>GKLHVGKMGFVVTMLKLIQKKLLDKTCDQVMEFSWSALW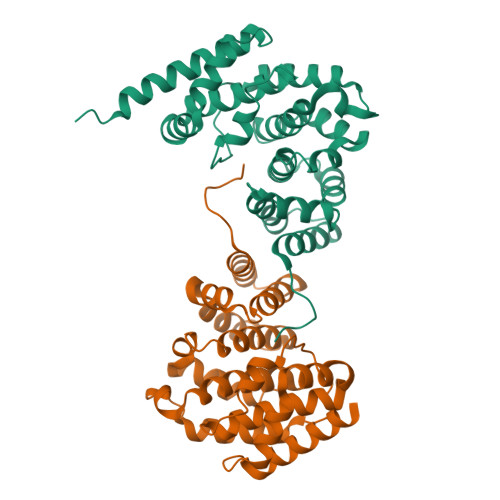NITDETPDNCEMFLNFNGMKLFLDCLKEFPEKQELHRNMLGLLGNVAEVKELRPQLMTSQFISVFSNLLESKADGIEVSYNACGVLSHIMFDGPEAWGVCEPQREEVEERMWAAIQSWDINSRRNINYRSFEPILRLLPQGISPVSQHWATWALYNLVSVYPDKYCPLLIKEGGMPLLRDIIKMATARQETKEMARKVIEHCSNFKEENMDTSR[2x]1-[(2-chlorophenyl)methyl]pyrazole-3,5-dicarboxylic acid | C12 H9 Cl N2 O4 | 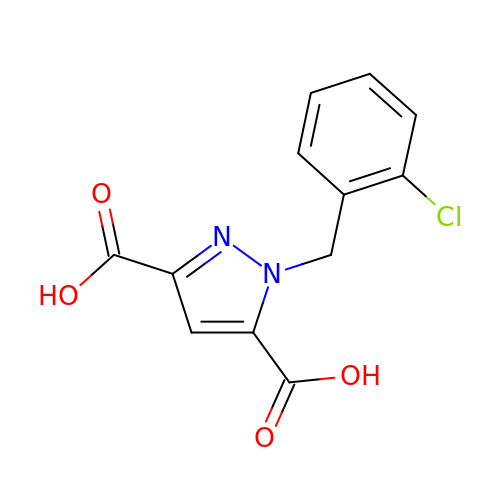DUFXLIZIBVXLGN-UHFFFAOYSA-N> IVGGYNCEENSVPYQVSLNSGYHFCGGSLINEQWVVSAGHCYKSRIQVRLGEHNIEVLEGNEQFINAAKIIRHPQYDRKTLNNDIMLIKLSSRAVINARVSTISLPTAPPATGTKCLISGWGNTASSGADYPDELQCLDAPVLSQAKCEASYPGKITSNMFCVGFLEGGKDSCQGDAGGPVVCNGQLQGVVSWGDGCAQKNKPGVYTKVYNY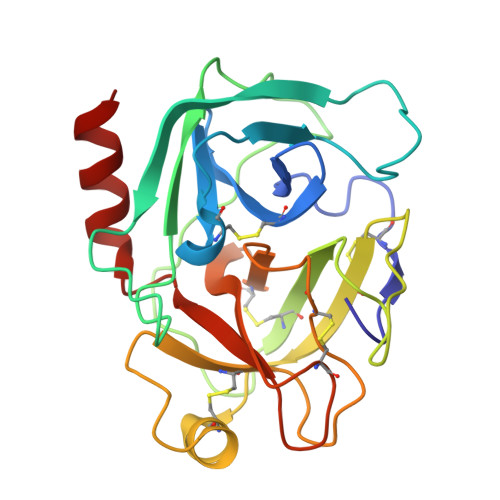VKWIKNTIAANS> MSAPSDQSQETRSPTSVGNTVAADVQTSVHDKPTGELKGSDGTGIHEATGLPIDKRGEVPTVQLERTAESIAKMMDLLRSEKFTAAAADAKLMLQQEFQNIVACAKNAPQMTVNAGRFYLGCNSTTAIIAGDTADGYEIEYSGKRIEGQCVVALEPLTITLSGSTSSTQDNSDSAKLFALAVSQVWGGASTVGIVAPMLQTVAQEQTFRARVERDSGFQHHAALTTVVTTIVGWLMHVGDSAAKRSRDGWLDHQTDFAVKGMLTPHIASGMDWAGVQTYSASAMETTTDRVRADYAGRMVVHSTLRKQTLRSRGTGDTTETENSGRYLLALPKCDAGVAAAALALTWGKPKLGGAGHANLTAVMSEAGVGYITGVNGTRATPHADTVFGREELVYLLGFALRHMADAQEQVIRNVLAQVASLFRPAACSAHEWMNVHGALMPKVSRPMNEPAFREVWNVANSSSDLQMIDRDKLNGEHFLRQLAQQITVNCTGTAMAIYQAVLAGPTGITDGDTTRLQKDLYHHLFQYATTTYADGVQVMQANTRMANKMVPPVNALAAWGLGSSMDSFTGPHCAYYFGLADAADGCFYSTTTGRTLSVYAVDVNHTSSDSYLAMAQLEPGLIATATGTGSTITTNVEAAGVVDGGLVTEGHVSLYTTISAQWNGLQREVYNWLLWHACKTEDSSHADIVGAEEVKSAVEWLSSNSVEAHRFRSSAGLGATEAAGSPGRRAWRLHHYDGQIFSNVIADTERHPYMRRLYTPSELRDARNDLFVVDRIWKIVMAMRAQLMLISVQEDGGRHQHSKHYFGEAAAIGVMGHGFTNLFAYCASTVHGGREARLISNCTDTPMYKKEANDLVPPMMKVAQLSTLLAHGGAWCNAVNMGGNSTSIGLSILGDGTMPLQTVPWTVNEITYLSEEGARHGIEAIIDTNGSVSVKVKMTMLEPRQRFCLYDDNKTSSYITAQESRTATYVTLKLGGTKNANTISGLVAHDYKLATTILASTYDKGRKTGLTLEDLQKVGGITGGQGMTGRGGGSSSGRGGRGRGGSSTGGAETIGD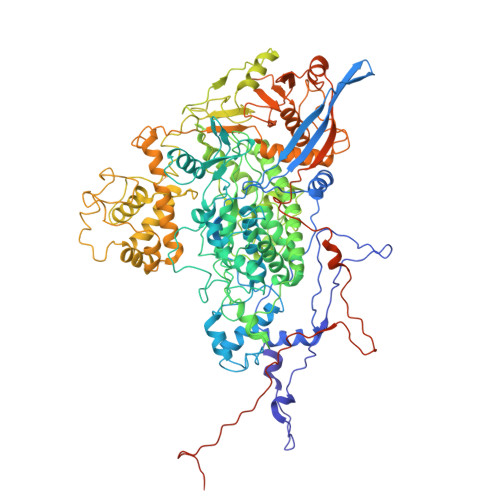SE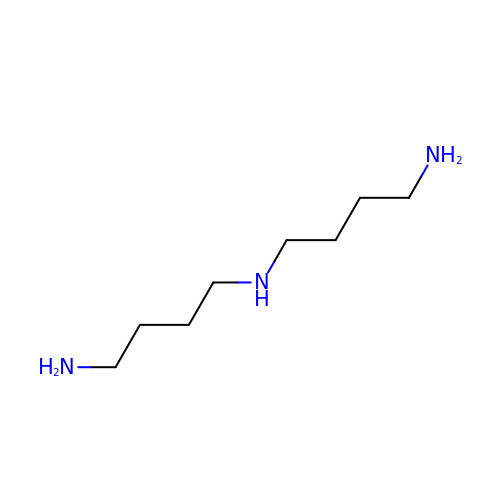sym-homospermidine | C8 H21 N3 | UODZHRGDSPLRMD-UHFFFAOYSA-N> GTHSLKYVYTGVSRGIDFPEFTAVGMVDDGQFMYFDSNSMKAVPKTEWIRQNEGADYWDRQTQVLIGAHQVFKDSIQIVMERFNQSKGVHTWQNMYGCELNDDGTTQGFYQ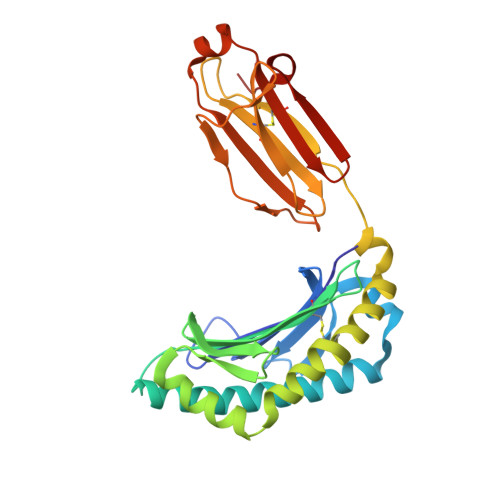YAYDGEDFVSLDKNTLTWTAANPQAVITKHKWEALAVAEQNKGYLENTCIEWLKKYVAYGKDTLERKVSPQVSLLQKDPSSPVTCHATGFYPSGVTITWQKNGQDHDEDVDLGELLPNEDGSFQRMSTLNVGPDEWKNNRFSCVVEHQDKTIRKTEDDIITNFD>[4x]MTDHVREADDANIDDLLGDLGGTARAERAKLVEWLLEQGITPDEIRATNPPLLLATRHLVGDDGTYVSAREISENYGVDLELLQRVQRAVGLARVDDPDAVVHMRADGEAAARAQRFVELGLNPDQVVLVVRVLAEGLSHAAEAMRYTALEAIMRPGATELDIAKGSQALVSQIVPLLGPMIQDMLFMQLRHMMETEAVNAGERAAGKPLPGARQVTVAFADLVGFTQLGEVVSAEEL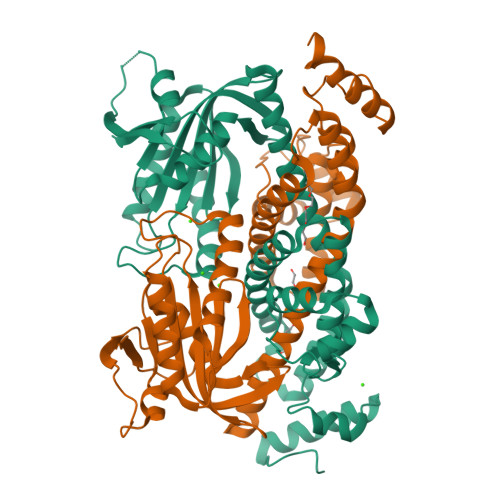GHLAGRLAGLARDLTAPPVWFIKTIGDAVMLVCPDPAPLLDTVLKLVEVVDTDNNFPRLRAGVASGMAVSRAGDWFGSPVNVASRVTGVARPGAVLVADSVREALGDAPEADGFQWSFAGPRRLRGIRGDVRLFRVRRGATRTGSGGAAQDDDLAGSSPGSRSHHHHHH>[2x]QSMQTGAFKIGVSMKTLSAPYFAAQMEAAKARGKELGYEVLATDAQGKLQKQISDVEDLVTRGVKLLIINPADSEGLVNAVNNASANGVKVVVIDSTLNPRANFVTQVQSSNSINGALVGHWVIEEVGNKSLKIALLSGEKGNPVGQERRLGVLSGIIEAQLRKFGKADLTVVGQGWGHWNDEGGLK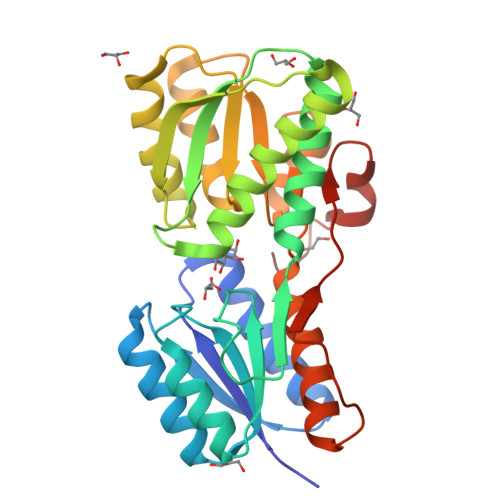AMEDLLVANKDINMVLGENDSMVLGARRAIESAGRTGILLVAAADAQKEALALIKQGKYGVTGLNDPALVARTAIDLGVKVVKGEVKDVPKQTLTTPAAITKGNVDKFYNPKAVF> PDALA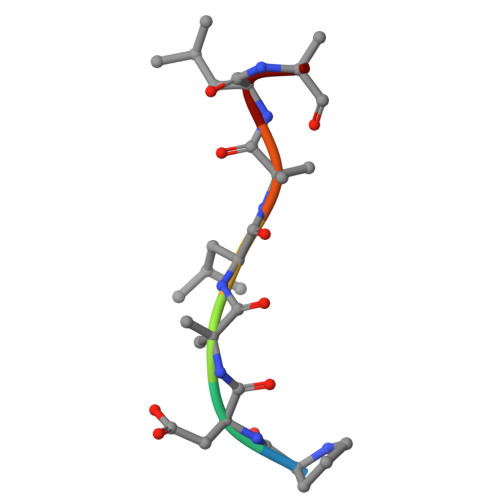LA> AEEAPRRVKLSQRQMQELKEAFTMIDQDRDGFIGMEDLKDMFSSLGRVPPDDELNAMLKECPGQLNFTAFLTLFGEKVSGTDPEDALRNAFSMFDEDGQGFIPEDYLKDLLENMGDNFSKEEIKNVWKDAPLKNKQFNYNKMVDIKGKAE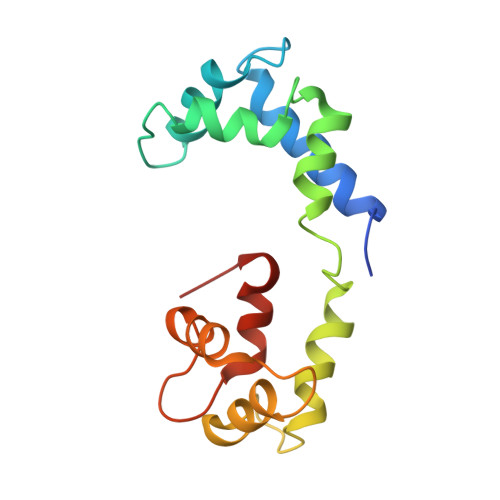DED> MKNFLLLTLILLTACNNSEENTQSIIKNDINKTIIDEEYVNLEPINQSNISFTKHSWVQTCGTQQLLTEQNKESISLSVVAPRLDDDEKYCFDFNGVSNKGEKYITKVTLNVVAPSLEVYVDHASLPTLQQLMDIIKSEEENPTAQRYIAWGRIVPTDEQMKELNITSFALINNHTPADLVQEIVKQAQTKHRLNVKLSSNTAHSFDNL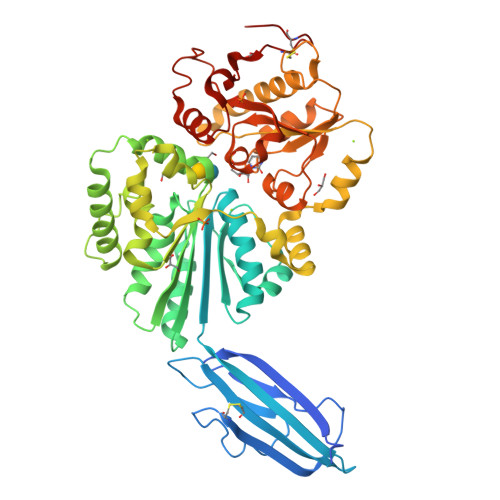VPILKELNSFNNVTVTNIDLYDDGSAEYVNLYNWRDTLNKTDNLKIGKDYLEDVINGINEDTSNTGTSSVYNWQKLYPANYHFLRKDYLTLEPSLHELRDYIGDSLKQMQWDGFKKFNSKQQELFLSIVNFDKQKLQNEYNSSNLPNFVFTGTTVWAGNHEREYYAKQQINVINNAINESSPHYLGNSYDLFFKGHPGGGIINTLIMQNYPSMVDIPSKISFEVLMMTDMLPDAVAGIASSLYFTIPAEKIKFIVFTSTETITDRETALRSPLVQVMIKLGIVKEENVLFWADLPNCETGVCIAV>[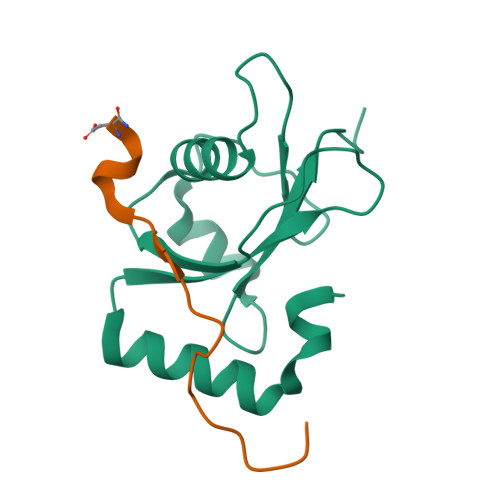2x]GSMKSTFKSEYPFEKRKAESERIADRFPNRIPVICEKAEKSDIPEIDKRKYLVPADLTVGQFVYVIRKRIMLPPEKAIFIFVNDTLPPTAALMSAIYQEHKDKDGFLYVTYSGENTFG;>[2x]ADSESEFENVANAGSMEQFETIDHKDLN> ADYDLKFGMNAGTSSNEYKAAE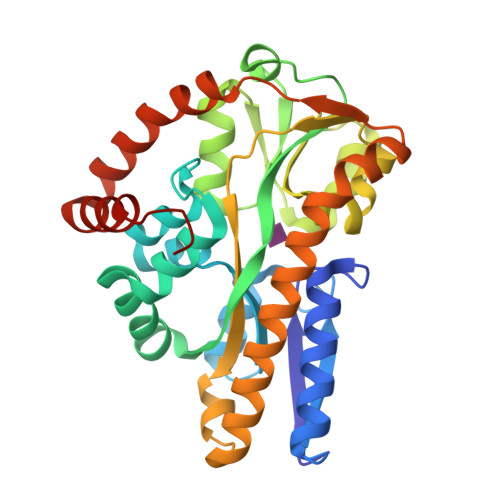MFAKEVKEKSQGKIEISLYPSSQLGDDRAMLKQLKDGSLDFTFAESARFQLFYPEAAVFALPYVISNYNVAQKALFDTEFGKDLIKKMDKDLGVTLLSQAYNGTRQTTSNRAINSIADMKGLKLRVPNAATNLAYAKYVGASPTPMAFSEVYLALQTNAVDGQENPLAAVQAQKFYEVQKFLAMTNHILNDQLYLVSNETYKELPEDLQKVVKDAAENAAKYHTKLFVDGEKDLVTFFEKQGVKITHPDLVPFKESMKPYYAEFVKQTGQKGESALKQIEAINPHHHHHH>MANIFLILFLFCFINFGNATPTTHNQDKTDKEEQYCVPNIEQDPQILLEQSLDAKDWALSNGLVKFVDVPTCPECGKKTKKMMTQFLPLSLYPSPFPRKLFQQAVDVQKAMLLLYFRASCDYEFLKEAHREVLNSELDNGIKKLVKRLDGMLSDGIRQPVAMFCQRADYMASQEDDGQYVLKQVEVNTGAIGSFGTTPRFSRLHRRMVSNAGIDASESVMPSDQTDTMAAETLYQAWLEFGNAEAVILFLHGSPNSHLMLESRQITHQLESISTERIKCRFITITEGLNRLKRDPNNFSLILDDKFVVAVVFDRLGGAVTKEEMDLNFVIDHSTAIKTPPYIFALSHTKRMQQVFTKPGMVEKFFNNPEEEHMAEAIRKVQTKGWAIGKDEDLTEDIIKKATENPHRYVLKNNGCSSNAADMFFNEDILKKLKTMAPADRDFYYLTEKLRPMVIKNHFVRPNMAPTLNLDATPELGIFGCLLGNMETGKVSYFSRTGHMMKSKLANVDEGGVWKGFSVYDSPYLV[2x]

Glutathione, the tri-peptide γ-L-glutamyl-cysteinyl-glycine, is the main low molecular weight thiol antioxidant in both plant and animal cells, often present at millimolar concentrations in vivo. It is synthesised in a two-step, ATP-dependent, process: glutamate-cysteine ligase (GCL) catalyses the formation of γ-glutamylcysteine (γ-EC) from glutamate and cysteine, followed by the addition of glycine by glutathione synthetase (GS) to form glutathione. Cyst nematodes have exploited a series of gene gain events to redeploy glutathione synthetase-like enzymes during parasitism, within the syncytial feeding cell formed in the host root. The most recent expansion has been coupled with a diversification of structure and biochemical function that has given rise to enzymes that are introduced into the host cell, and likely possess novel substrate specificities.

To explore the catalytic capacity of nematode GS-like genes, the G. pallida representative of Clade 1 (Gpa-gss1), one representative from Clade 2 (Gpa-gss5) and a number from Clade 3 (Gpa-gss12, Gpa-gss17, Gpa-gss22, Gpa-gss24 and Gpa-gss30) were heterologously expressed in, and their proteins purified from, bacteria. Remarkably, each stage of the evolutionary process that gave rise to GS-like effectors has witnessed at least a 10-fold reduction in apparent glutathione synthetic rate, such that Clade 3 GS-like proteins have not retained canonical enzyme activity. In contrast, none of the Clade 3 GS-like effectors accepted any of the tested terminal amino acid substrates in combination with the γ-EC backbone. One possible explanation for this is that Clade 3 GS-like effectors represent a novel diversification at the site of the di-peptide acceptor. However, the glutamate of the di-peptide is exclusively coordinated by interactions with charged side chains of residues in the binding pocket (R, E, 2xQ, N, and Y). All six of these positions are substituted in Gpa-GSS22 and Gpa-GSS30, thus suggesting that the lack of canonical activity is because γ-EC is not accepted despite the potential for cysteine to be accommodated. Variability in the glutamate portion of the di-peptide binding pocket is ubiquitous in G. pallida Clade 3 GS: of the 24 GS-like effectors there are 21 different amino acid compositions in these 6 positions, not one of which is canonical. Coupled with the high degree of conservation in the ATP-binding pocket, the functioning ATP-grasp fold, and the perfect conservation of a catalytic residue, these data support the hypothesis that the loss of canonical glutathione synthetic activity is associated with a gain of non-canonical activity.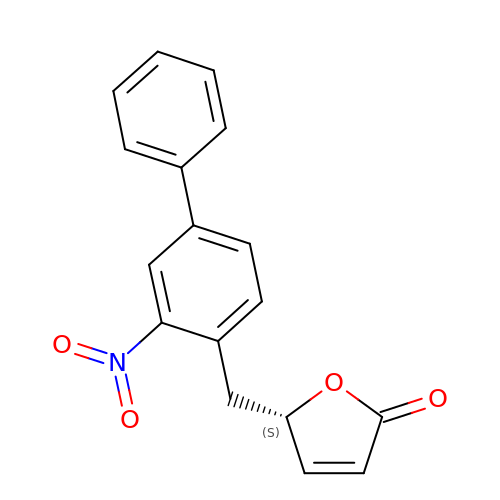(2~{S})-2-[(2-nitro-4-phenyl-phenyl)methyl]-2~{H}-furan-5-one | C17 H13 N O4 | RCYKWQHJOBNQFZ-OAHLLOKOSA-N> MSELFSERIPPQSIEAEQAVLGAVFLDPAALVPASEILIPEDFYRAAHQKIFHAMLRVADRGEPVDLVTVTAELAASEQLEEIGGVSYLSELADAVPTAANVEYYARIVEEKSVLRRLIRTATSIAQDGYTREDEIDVLLDEADRKIMEVSQRKHSGAFKNIKDILVQTYDNIEMLHNRDGEITGIPTGFTELDRMTSGFQRSDLIIVAARPSVGKTAFALNIAQNVATKTNENVAIFSLEMS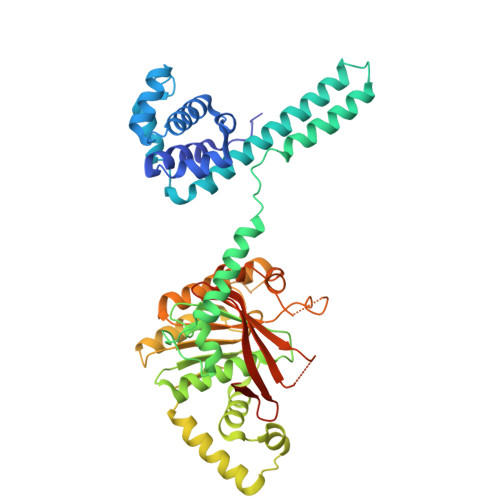AQQLVMRMLCAEGNINAQNLRTGKLTPEDWGKLTMAMGSLSNAGIYIDDTPSIRVSDIRAKCRRLKQESGLGMIVIDYLQLIQGSGRSKENRQQEVSEISRSLKALARELEVPVIALSQLSRSVEQRQDKRPMMSDIRESGSIEQDADIVAFLYRDDYYNKDSENKNIIEIIIAKQRNGPVGTVQLAFIKEYNKFVNLERRFDEAQIPPGA>SLMADEIAKAQVARPGGDTIFGKIIRKEIPAKIIFEDDRCLAFHDISPQAPTHFLVIPKKHISQISVAEDDDESLLGHLMIVGKKCAADLGLNKGYRMVVNEGSDGG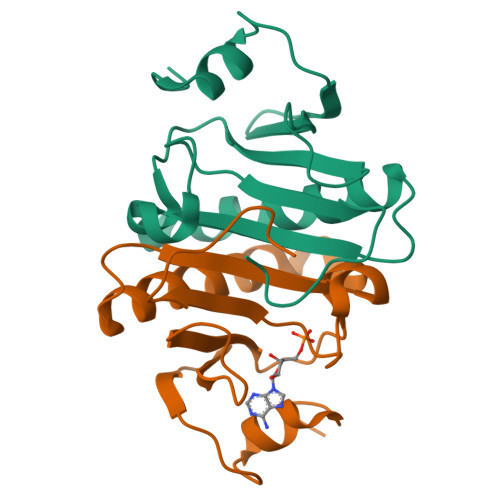QSVYHVHLHVLGGRQMHWPPG[2x]> MHHHHHHLILAPMVRVGTLPMRLLALDYGADIVYCEELIDLKMIQCKRVVNEVLSTVDFVAPDDRVVFRTCEREQNRVVFQMGTSDAERALAVARLVENDVAGIDVNMGCPKQYSTKGGMGAALLSDPDKIEKILSTLVKGTRRPVTCKIRILPSLEDTLSLVKRIERTGIAAIAVHGRKREERPQHPVSCEVIKAIADTLSIPVIANGGSHDHIQQYSDIEDFRQATAASSVMV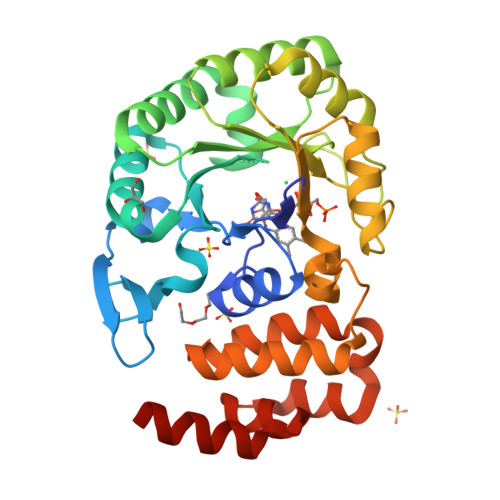ARAAMWNPSIFLKEGLRPLEEVMQKYIRYAVQYDNHYTNTKYCLCQMLREQLKSPQGRLLHAAKSSREICEAFGLGAFYEETTQELDAQQAR>GPNCAPGKVKLFRASEPILSVLMWGVNHTINELSNVPVPVMLMPDDFKAYSKIKVDNHLFNKENLPSRFKFKEYCPMVFRNLRERFGIDDQDYQNSVTRSAPINSDSQGRCGTRFLTTYDRRFVIKTVSSEDVAEMHNILKKYHQFIVECHGNTLLPQFLGMYRLTVDGVETYMVVTRNVFSHRLTVHRKYDLKGSTVAREASDKEKAKDLPTFKDNDFLNEGQKLHVGEESKKNFLEKLKRDVEFLAQLKIMDYSLLVGIHDVDRAEQEEMEVEERAEDEECENDGVGGNLLCSYGTPPDSPGNLLSFPRFFGPGEFDP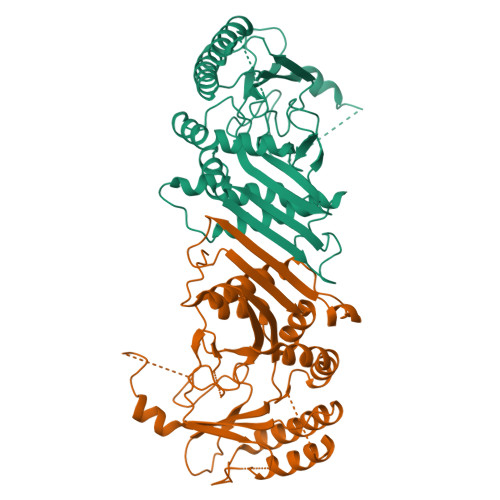SVDVYAMKSHESSPKKEVYFMAIIDILTPYDTKKKAAHAAKTVKHGAGAEISTVNPEQYSKRFNEFMSNILT[2x]>[2x]GGAAUCAAUAGUAGUUAACCCUCUCUUCCGAAGCGAGCCGGGGGCGGUGGGAGCCCGGUGAAGACGGUUAAUGAAACGGCAGUUCC;>[2x]GCGG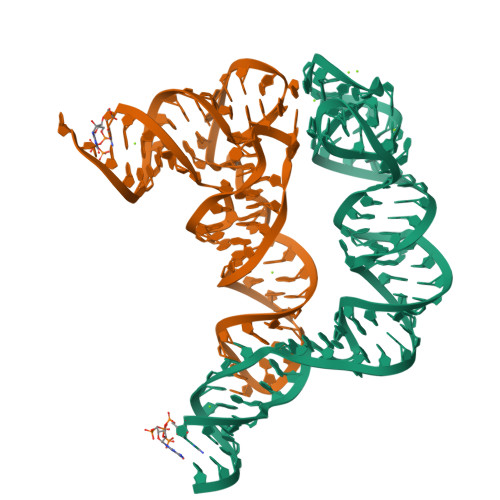AAGUAGUUCAGUGGUAGAACACCACCUUGCCAAGGUGGGGGUCGCGGGUUCGAGUCCCGUCUUCCGCUCCA>[4x]AAQSVDIHKDQIIFSEGDAGDCAYIIEKGRVLIYLTKDKEEIPLTILGEGEI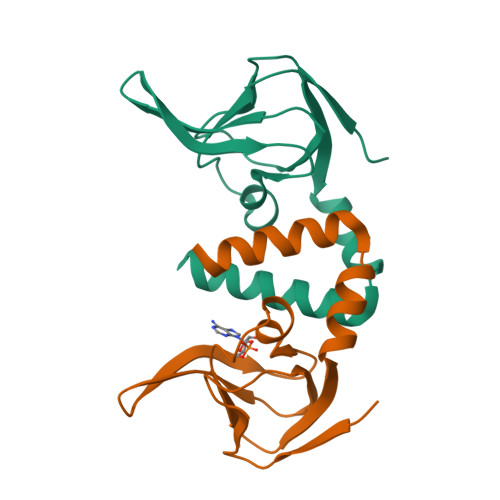FGEMALIDNQNRSASVRALEDVRLAIVTKQQVLERVSTADKVVQLLMRVLLKRLRRKNI>THPDISVDVLVIGAGPTGLGAAKRLNQIDGPSWMIVDSNETPGGLASTDVTPEGFLYDVGGHVIFSHYKYFDDCLDEALPKEDDWYTHQRISYVRCQGQWVPYP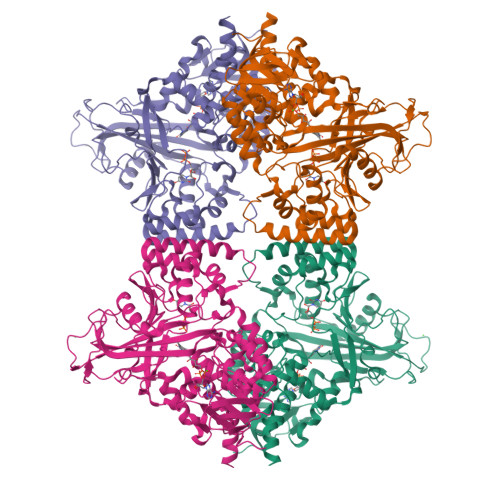FQNNISMLPKEEQVKCIDGMIDAALEARVANTKPKTFDEWIVRMMGTGIADLFMRPYNFKVWAVPTTKMQCAWLGERVAAPNLKAVTTNVILGKTAGNWGPNATFRFPARGGTGGIWIAVANTLPKEKTRFGEKGKVTKVNANNKTVTLQDGTTIGYKKLVSTMAVDFLAEAMNDQELVGLTKQLFYSSTHVIGVGVRGSRPERIGDKCWLYFPEDNCPFYRATIFSNYSPYNQPEASKKLPTMQLADGSRPQSTEAKEGPYWSIMLEVSESSMKPVNQETILADCIQGLVNTEMLKPTDEIVSTYHRRFDHGYPTPTLEREGALTQILPKLQDKDIWSRGRFGSWRYEVGNQDHSFMLGVEAVDNIVNGAVELTLNYPDFVNGRQNTERRLVDGAQVFAKSKAQL[8x]>[4x]MN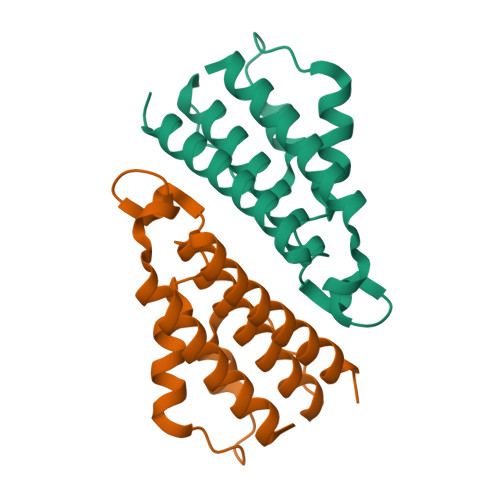RARDWLEQARHNLRHAQGSLGLGDYAWACFAAQQAAEAALKGLHLARGQVAWGHSILDLLADLPEDVDVPEDLVEAAKVLDKYYIPTRYPDAHPAGPAARHYTRLEAEEALDLAQKILAFVEEKL> NCSKIHLSTKLLAVDFPAHFVKSISCQICEHILADPVETSCKHLFCRICILRCLKVMGSYCPSCRYPCFPTDLESPVKSFLNILNSLMVKCPAQDCNEEVSLEKYNHHVSSHKESKETLVHINKGGRPRQHLLSLTRRAQKHRLRELKIQVKEFADKEEGGDVKAVCLTLFLLALRARNEHRQADELEAIMQGRGSGLQPAVCLAIRVNTFLSCSQYHKMYRTVKAITGRQIFQPLHALRNAEKVLLPGYHPFEWQPPLKNVSSRTDVGIIDGLSGLASSVDEYPVDTIAKRFRYDSALVSALMDMEEDILEGMRSQDLDDYLNGPFTVVVKESCDGMGDVSEKHGSGPAVPEKAVRFSFTVMRITIEHGSQNVKVFEEPKPNSELCCKPLCLMLADESDHETLTAILSPLIAEREAMKSSELTLEMGGIPRTFKFIFRGTGYDEKLVREVEGLEASGSVYICTLCDTTRLEASQNLVFHSITRSHAENLQRYEVWRSNPYHESVEELRDRVKGVSAKPFIETVPSIDALHCDIGNAAEFYKIFQLEIGEVYKHPNASKEERKRWQATLDKHLRKRMNLKPIMRMNGNFARKLMTQETVDAVCELIPSEERHEALRELMDLYLKMKPVWRSSCPAKECPESLCQYSFNSQRFAELLSTKFKYRYEGKITNYFHKTLAHVPEIIERDGSIGAWASEGNQSGNKLFRRFRKMNARQSKCYEMEDVLKHHWLYTSKYLQKF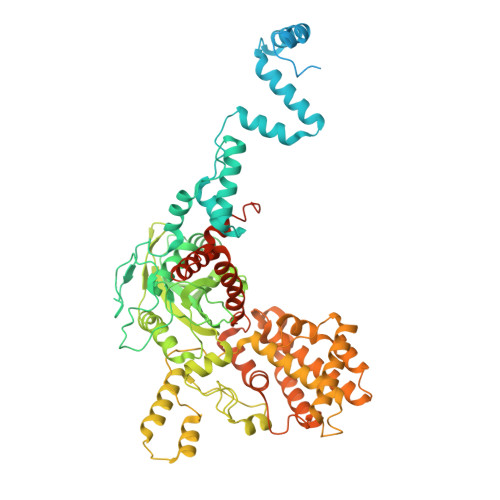MNAHNALKSSGFTMNSKETLGDPLGIEDSLESQDSMEF>MGQIFTVQELKERAKVFAKPIGASYQGILDQLDLVHQAKGRDQIAASFELNKKINDYIAEHPTSGRNQAL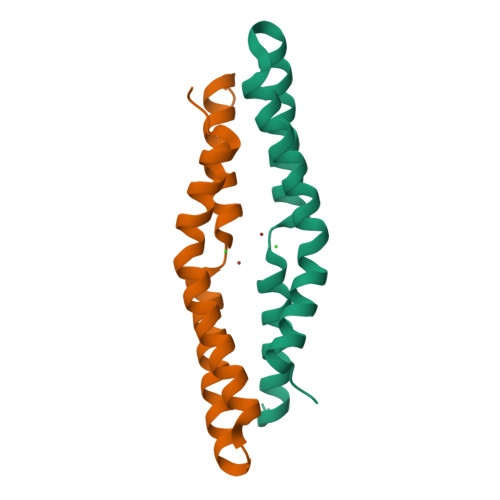TQLKEQVTSALGLEHHHHHH[2x]The HCV NS3/4A protease – a chymotrypsin-like serine protease – is a prime therapeutic target that cleaves four known sites along the virally encoded polyprotein. The NS3/4A protease also hydrolyzes two human proteins, TRIF and MAVS, which are part of the innate immune system, thereby confounding the innate immune response to viral infection. In this study, we report that four chemically representative protease inhibitors – telaprevir, danoprevir, vaniprevir and MK-5172 – exhibit distinct susceptibilities to the protease variants R155K, A156T and D168A. To elucidate the underlying mechanism by which chemically diverse inhibitors bind to the wild-type protease and drug-resistant variants, crystal structures were determined for 16 inhibitor-protease complexes. These complexes include wild-type protease and resistant variants R155K, D168A and A156T each bound to telaprevir, danoprevir, vaniprevir and MK-5172, with resolutions ranging from 1.10–2.50 Å; S139A protease variants were used except for telaprevir, which requires covalent bond formation with the serine 139 for efficient binding.

The most potent of the NS3/4A protease inhibitors is MK-5172. Against wild-type protease, macrocyclic inhibitors danoprevir, vaniprevir and MK-5172 exhibited antiviral potencies in the sub nM range (IC50 = 0.24, 0.34 and 0.11 nM, respectively), while telaprevir potency was significantly lower (IC50 = 1030 nM), consistent with previous reports. The acylsulfonamide groups of danoprevir, vaniprevir and MK-5172 were also positioned in the oxyanion hole, hydrogen bonding with the same set of backbone amide nitrogens, as observed previously for the TMC435 and danoprevir structures. Meanwhile the Nε nitrogen of H57 interacted with the sulfonamide nitrogen in these complexes, suggesting that the Nε atoms were deprotonated. In contrast, MK5172 adopted a novel conformation with the ether-linked P2 quinoxaline moiety not interacting extensively with R155 and D168, but stacking instead against H57 and D81 of the catalytic triad. Notably MK-5172, with an ether-linked P2 quinoxaline moiety, while protruding from the substrate envelope, stacked against the catalytic triad, avoiding direct van der Waals contact with R155 and D168. Unlike in the danoprevir and vaniprevir complexes with wild type, in the MK-5172-wild-type complex the P2 quinoxaline moiety did not stack on R155 and interacted less with D168 and the electrostatic network involving these residues. We report here, for the first time, a novel binding conformation for MK-5172 in which the P2 quinoxaline moiety binds far from the S2 subsite and instead stacks against the catalytic residues H57 and D81. MK-5172 has a unique barrier to resistance, as neither catalytic residue (H57 or D81) can tolerate mutation. The high potency of MK-5172, for example, derives from interactions with the essential catalytic triad residues, which cannot mutate without severely disrupting viral fitness.

>GSHMASMKKKGSVVIVGRINLSGDTAYAQQTRGEEGCQETSQTGRDKNQVEGEVQIVSTATQTFLATSINGVLWTVYHGAGTRTIASPKGPVTQMYTNVDKDLVGWQAPQGSRSLTPCTCGSSDLYLVTRHADVIPVRRRGDSRGSLLSPRPISYLKGSAGGPLLCPAGHAVGIFRAAVSTRGVAKAVDFIPVESLETTMRSP[4x]>[4x]VNLPGSKSVSNRALLLAALASGTTRLTNLLDSDDIRHMLNALTKLGVNYRLSADKTTCEVEGLGQAFHTTQPLEL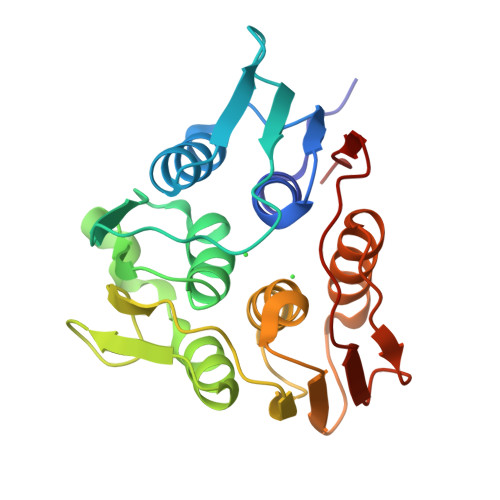FLGNAGTAMRPLAAALCLGQGDYVLTGEPRMKERPIGHLVDALRQAGAQIEYLEQENFPPLRIQGTGLQAGTVTIDGSISSQFLTAFLMSAPLAQGKVTIKIVGELVSKPYIDITLHIMEQFGVQVINHDYQEFVIPAGQSYVSPGQFLVEGD> LSGDAVQKMLGHCTFEPAEPKAAKNTYTAERFIWLTKLNNLRILEQG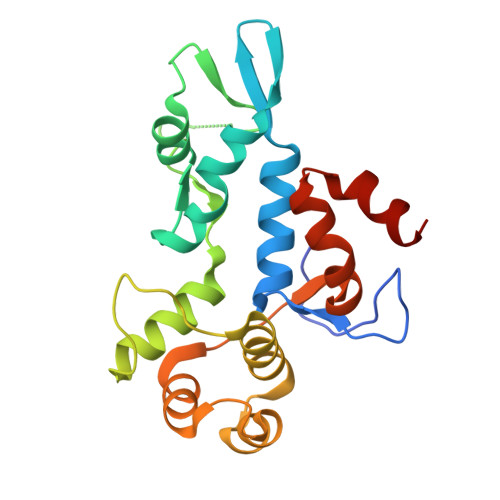SERPLTDTERATLMDEPYRKSKLTYAQARKLLGLEDTAFFKGLRYGKDNAEASTLMEMKAYHAISRALEKEGLKDKKSPLNLSPELQDEIGTAFSLFKTDEDITGRLKDRIQPEILEALLKHISFDKFVQISLKALRRIVPLMEQGKRYDEACAEIYGDHY> LPTLGPGWQRQNPDPPVSRTRSLLLDAASGQLRLEDGFHPDAVAWANLTNAIRETGWAYLDLSTNGRYNDSLQAYAAGVVEASVSEELIYMHWMNTVVNYCGPFEYEVGYCEKLKNFLEANLEWMQREMELNPDSPYWHQVRLTLLQLKGLEDSYEGRLTFPTGRFTIKPLGFLLLQISGDLEDLEPALNKTNTKPSLGSGSCSALIKLLPGGHDLLVAHNTWNSYQNMLRIIKKYRLQFREGPQEEYPLVAGNNLVFSSYPGTIFSGDDFYILGSGLVTLETTIGNKNPALWKYVQPQGCVLEWIRNVVANRLALDGATWADVFKRFNSGTYNNQWMIVDYKAFLPNGPSPGSRVLTILEQIPGMVVVADKTAELYKTTYWASYNIPYFETVFNASGLQALVAQYGDWFSYTKNPRAKIFQRDQSLVEDMDAMVRLMRYNDFLHDPLSLCEACNPKPNAENAISARSDLNPANGSYPFQALHQRAHGGIDVKVTSFTLAKYMSMLAASGPTWDQCPPFQWSKSPFHSMLHMGQPDLWMFSPIRVPWDGRGSHHHHHHG

In order to gain insight into the function and the post-translational maturation process of the glycosylated 66.3 kDa protein, three crystal structures were determined that represent different maturation states. These structures demonstrate that the 28 kDa and 40 kDa fragment which have been derived by a proteolytic cleavage remain associated. The core αββα sandwich fold and a cysteine residue at the N-terminus of the 40 kDa fragment (C249) classify the 66.3 kDa protein as a member of the structurally defined N-terminal nucleophile (Ntn) hydrolase superfamily. However, the structural classification of the 66.3 kDa protein as an Ntn hydrolase implies a hydrolytic activity on a kind of non-peptide amide bond as commonly observed for Ntn hydrolases.

Superposition of the three refined structures of the 66.3 kDa protein reveals only slight variations in the overall conformation. The major difference between the three structures concerns a linker peptide of about ten amino acids N-terminal of C249. The most significant difference concerns the peptide bond connecting residues S248 and C249. Upon cleavage, the conformation of S248 and C249 changes significantly. The cleavage is additionally accompanied by slight changes of the torsion angles of the adjacent residue S248, which is within the allowed region of a left-handed α-helix before and in the core β-strand region of the Ramachandran plot after the cleavage. Based on these observations, we assume that the processing step which gives rise to the 28 kDa and 40 kDa fragments starts with a cleavage between S248 and C249. All functional Ntn hydrolases known so far are activated by autocatalytic cleavage.>PIELLPETPSQTAGPYVHIGLALEAAGNPTRDQEIWNRLAKPDAPGEHILLLGQVYDGNGHLVRDSFLEVWQADANGEYQDAYNLENAFNSFGRTATTFDAGEWTLHTVKPGVVNNAAGVPMAPHINISLFARGINIHLHTRLYFDDEAQANAKCPVLNLIEQPQRRETLIAKRCEVDGKTAYRFDIRIQGEGETVFFDF[6x];>[6x]PAQDNSRFVIRDRNWHPKALTPDYKTSIARSPRQALVSIPQSISETTGPNFSHLGFGAHDHDLLLNFNNGGLPIGERIIVAGRVVDQYGKPVPNTLVEMWQANAGGR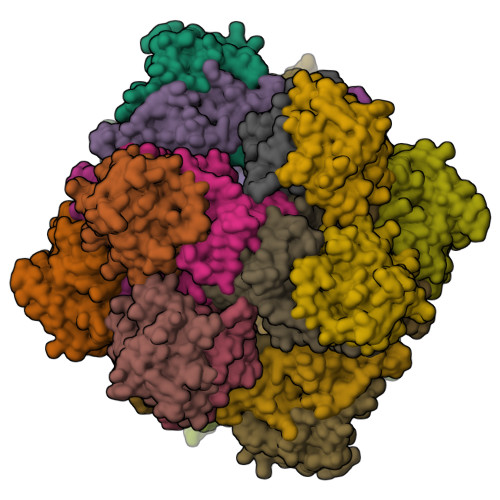ERHKNDRYLAPLDPNFGGVGRCLTDSDGYYSFRTIKPGPYPWRNGPNDWRPAHIHFGISGPSIATKLITQLYFEGDPLIPMCPIVKSIANPEAVQQLIAKLDMNNANPMDCLAYRFDIVLRGQRKTHFENC> MEYEWKPDEQGLQQILQLLKESQSPDTTIQRTVQQKLEQLNQYPDFNNYLIFVLTKLKSEDEPTRSLSGLILKNNVKAHFQNFPNGVTDFIKSECLNNIGDSSPLIRATVGILITTIASKGELQNWPDLLPKLCSLLDSEDYNTCEGAFGALQKICEDSAEILDSDVLDRPLNIMIPKFLQFFKHSSPKIRSHAVACVNQFIISRTQALMLHIDSFIENLFALAGDEEPEVRKNVCRALVMLLEVRMDRLLPHMHNIVEYMLQRTQDQDENVALEACEFWLTLAEQPICKDVLVRHLPKLIPVLVNGMKYSDIDIILLKGDVEGGSGGDDTISDWNLRKCSAAALDVLANVYRDELLPHILPLLKELLFHHEWVVKESGILVLGAIAEGCMQGMIPYLPELIPHLIQCLSDKKALVRSITCWTLSRYAHWVVSQPPDTYLKPLMTELLKRILDSNKRVQEAACSAFATLEEEACTELVP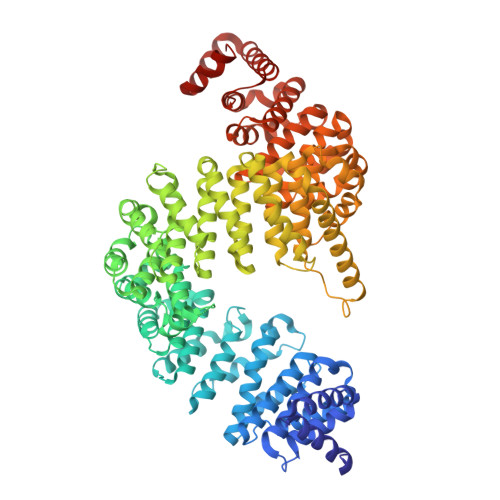YLAYILDTLVFAFSKYQHKNLLILYDAIGTLADSVGHHLNKPEYIQMLMPPLIQKWNMLKDEDKDLFPLLECLSSVATALQSGFLPYCEPVYQRCVNLVQKTLAQAMLNNAQPDQYEAPDKDFMIVALDLLSGLAEGLGGNIEQLVARSNILTLMYQCMQDKMPEVRQSSFALLGDLTKACFQHVKPCIADFMPILGTNLNPEFISVCNNATWAIGEISIQMGIEMQPYIPMVLHQLVEIINRPNTPKTLLENTAITIGRLGYVCPQEVAPMLQQFIRPWCTSLRNIRDNEEKDSAFRGICTMISVNPSGVIQDFIFFCDAVASWINPKDDLRDMFCKILHGFKNQVGDENWRRFSDQFPLPLKERLAAFYGV> LMITSFANPRVAQAFVDYMATQGVILTIQQHNQSDVWLADESQAERVRAELARFLENPADPRYLAASWQA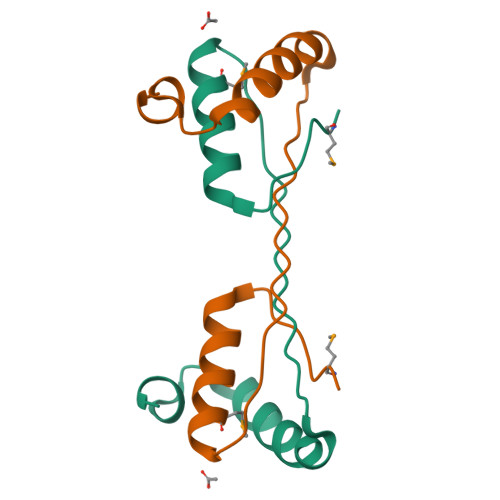GHTENLYFQ>GASMQPDMSLNVIKMKSSDFLESAELDSGGFGKVSLAFHRTQGLMIMKTVYKGPNCIEHNEALLEEAKMMNRLRHSRVVKLLGVIIEEGKYSLVMEYMEKGNLMHVLKAEMSTPLSVKGRIILEIIEGMAY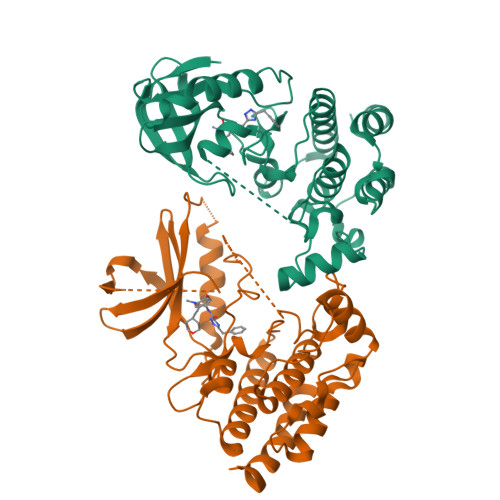LHGKGVIHKDLKPENILVDNDFHIKIADLGLASFKMWSKLNNEEHNELREVDGTAKKNGGTLYYMAPEHLNDVNAKPTEKSDVYSFAVVLWAIFANKEPYENAIAEQQLIMAIKSGNRPDVDDITEYCPREIISLMKLCWEANPEARPTFPGIEEKFRPFYLSQLE[2x]> TVGAVALDLDGNLAAATSTGGMTNKLPGRVGDSPLVGAGCYANN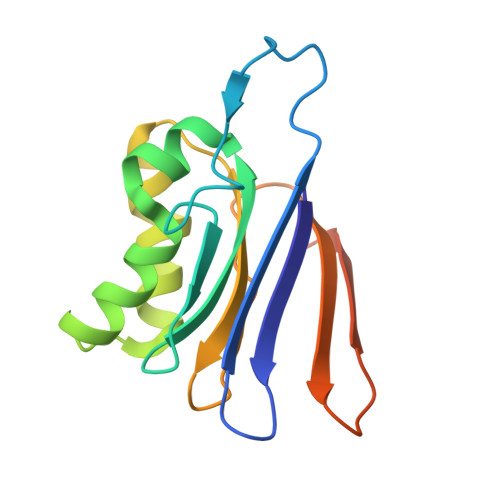ASVAVSCTGTGEVFIRALAAYDIAALMDYGGLSLAEACERVVMEKLPALGGSGGLIAIDHEGNVALPFNTEGMYRAWGYAGDTPTTGIYREKGDTVATQHSIE> GAEAEAPSAVPDAA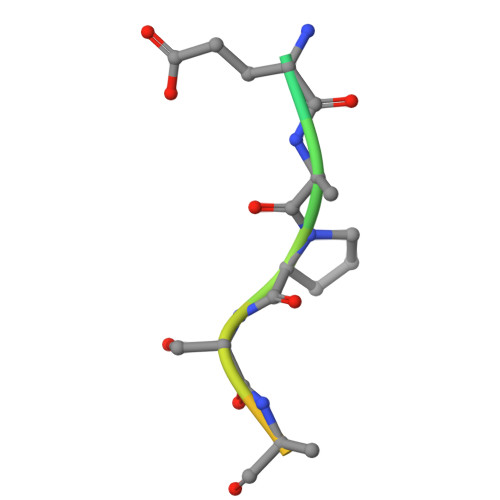G> MVYSYTEKKRIRKDFGKRPQVLDVPYLLSIQLDSFQKFIEQDPEGQYGLEAAFRSVFPIQSYSGNSELQYVSYRLGEPVFDVQECQIRGVTYSAPLRVKLRLVIYEREAPEGTVKDIKEQEVYMGEIPLMTDNGTFVINGTERVIVSQLHRSPGVFFDSDKGKTHSSGKVLYNARIIPYRGSWLDFEFDPKDNLFVRIDRRRKLPATIILRALNYTTEQILDLFFEKVIFEIRDNKLQMELVPERLRGETASFDIEANGKVYVEKGRRITARHIRQLEKDDVKLIEVPVEYIAGKVVAKDYIDESTGELICAANMELSLDLLAKLSQSGHKRIETLFTNDLDHGPYISETLRVDPTNDRLSALVEIYRMMRPGEPPTREAAESLFENLFFSEDRYDLSAVGRMKFNRSLLREEIEGSGILSKDDIIDVMKKLIDIRNGKGEVDDIDHLGNRRIRSVGEMAENQFRVGLVRVERAVKERLSLGDLDTLMPQDMINAKPISAAVKEFFGSSQLSQFMVQNNPLSEITHKRRISALGPGGLTRERAGFEVRDVHPTHYGRVCPIETPEGPNIGLINSLSVYAQTNEYGFLETPYRKVTDGVVTDEIHYLSAIEEGNYVIAQANSNLDEEGHFVEDLVTCRSKGESSLFSRDQVDYMDVSTQQVVSVGASLIPFLEHDDANRALMGANMQRQAVPTLRADKPLVGTGMERAVAVDSGVTAVAKRGGVVQYVDASRIVIKVNEDEMYPGEAGIDIYNLTKYTRSNQNTCINQMPCVSLGEPVERGDVLADGPSTDLGELALGQNMRVAFMPWNGYNFEDSILVSERVVQEDRFTTIHIQELACVSRDTKLGPEEITADIPNVGEAALSKLDESGIVYIGAEVTGGDILVGKVTPKGETQLTPEEKLLRAIFGEKASDVKDSSLRVPNGVSGTVIDVQVFTRDGVEKDKRALEIEEMQLKQAKKDLSEELQILEAGLFSRIRAVLVAGGVEAEKLDKLPRDRWLELGLTDEEKQNQLEQLAEQYDELKHEFEKKLEAKRRKITQGDDLAPGVLKIVKVYLAVKRRIQPGDKMAGRHGNKGVISKINPIEDMPYDENGTPVDIVLNPLGVPSRMNIGQILETHLGMAAKGIGDKINAMLKQQQEVAKLREFIQRAYDLGADVRQKVDLSTFSDEEVMRLAENLRKGMPIATPVFDGAKEAEIKELLKLGDLPTSGQIRLYDGRTGEQFERPVTVGYMYMLKLNHLVDDKMHARSTGSYSLVTQQPLGGKA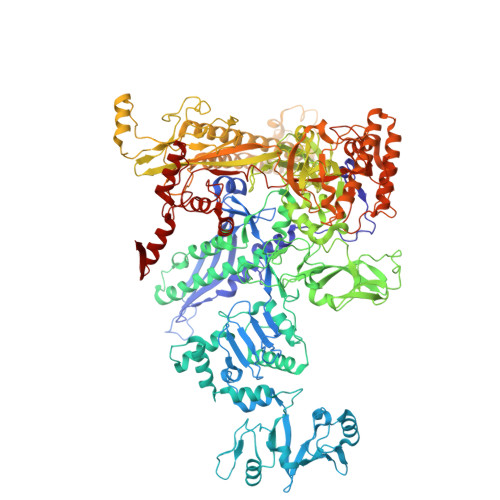QFGGQRFGEMEVWALEAYGAAYTLQEMLTVKSDDVNGRTKMYKNIVDGNHQMEPGMPESFNVLLKEIRSLGINIELEDE> XS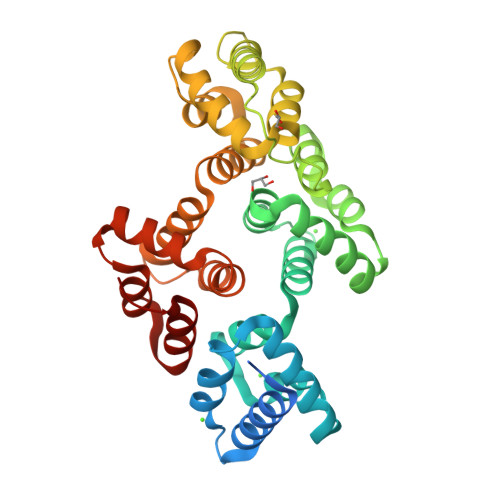TVHEILCKLSLEGDHSTPPSAYGEVKAYTNFDAERDALNIETAIKTKGVDEVTIVNILTNRSNEQRQDIAFAYQRRTKKELASALKSALSGHLETVILGLLKTPAQYDASELKASMKGLGTDEDSLIEIICSRTNQELQEINRVYKEMYKTDLEKDIISDTSGDFRKLMVALAKGRRAEDGSVIDYELIDQDARDLYDAGVKRKGTDVPKWISIMTERSVPHLQKVFDRYKSYSPYDMLESIRKEVKGDLENAFLNLVQCIQNKPLYFADRLYDSMKGKGTRDKVLIRIMVSRSEVDMLKIRSEFKRKYGKSLYYYIQQDTKGDYQKALLYLCGGDD>[2x]GSTSAQEWQPVYPMSQLSFDRILKKDLVQGEHLGRGTRTHIYSGTLMDYKDDEGTSEEKKIKVILKVLDPSHRDISLAFFEAASMMRQVSHKHIVYLYGVCVRDVENIMVEEFVEGGPLDLFMHRKSDVLTTPWKFKVAKQLASALSYLEDKDLVHGNVCTKNLLLAREGIDSECGPFIKLSD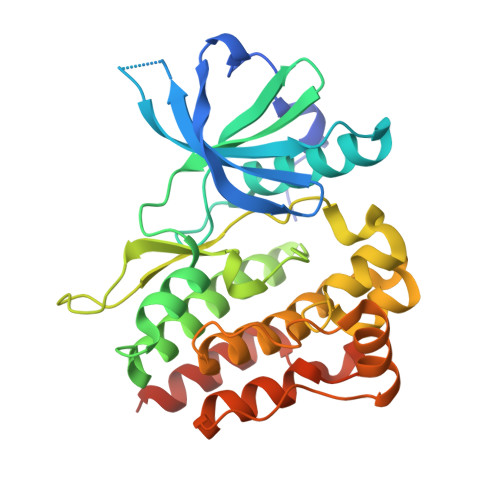PGIPITVLSRQECIERIPWIAPECVEDSKNLSVAADKWSFGTTLWEICYNGEIPLKDKTLIEKERFYESRCRPVTPSCKELADLMTRCMNYDPNQRPFFRAIMRDINKLEEQNPDIVSEKK>[2x]GASAVLFPCKYATTGCSLTLHHTEKPEHEDICEYRPYSCPCPGASCKWQGSLEAVMSHLMHAHKSITTLQGEDIVFLATDINLPGAVDWVMMQSCFGHHFM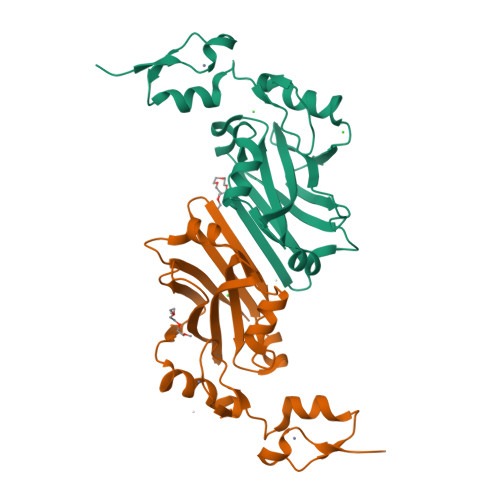LVLEKQEKYEGHQQFFAIVLLIGTRKQAENFAYRLELNGNRRRLTWEATPRSIHDGVAAAIMNSDCLVFDTAIAHLFADNGNLGINVTIST> QFAKPEDAVKYRQSALTLMASHFGRMTPVVKGQAPYDAAQIKANVEVLKTLSALP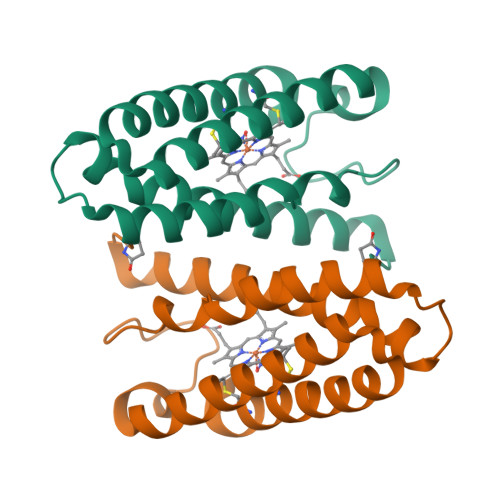WAAFGPGTEGGDARPEIWSDAASFKQKQQAFQDNIVKLSAAADAGDLDKLRAAFGDVGASCKACHDAYFKKK>PGVERTDITYNLTSDIDAAAYLEELKQNPIINNKIMNPVGQCESLMTPVSNFMNEKGFDNIRYRGIFIWDKPTEEIPTNHFAVVGNKEGKDYVFDVSAHQFENRGMSNLNGPLILSADEWVCKYRMATRRKLIYYTDFSNSSIAANAYDALPRELESESMAGKVFVTSPRWFNTFKKQKYSLIGKM[2x]

SseI is secreted into host cells by Salmonella and contributes to the establishment of systemic infections. SseI (also called SrfH) is an SPI-2-translocated protein that has been directly linked to systemic infection. The C-terminal domain (∼140–322) of SseI contains its catalytic function and shows some sequence similarity (19% identity over a 88-amino-acid stretch) to Pasteurella multocida toxin (PMT or ToxA), which causes atrophic rhinitis in swine. Based on its structural matches, SseI is a member of a particular subgroup (clan CA) of the cysteine protease superfamily.

Crystals of reductively methylated SeMet-derivative and native forms of SseI (37–322) were grown as described and their structures were solved using SAD and molecular replacement, respectively. The native crystals diffracted to 2.05 Å resolution and belonged to a different space group (P212121) to the SeMet-derivative crystals (P41212). The native structure was solved using the SeMet-derivative structure as a starting model and showed two molecules of the protein per asymmetric unit. No density was observed for the first 12 and the last nine residues of each molecule. The dimer is linked by a disulfide bond between Cys258 of each chain on the opposite face of the molecule to the catalytic Cys176. The dimer is likely to be a crystal artifact since the C-terminal domain purifies as a monomer on size-exclusion chromatography. The SeMet protein was purified using 10 mM DTT instead of 2 mM DTT to prevent Se oxidation, which may explain why it did not crystallize as a disulfide-linked dimer under these reducing conditions. The chain backbone in the native structure did not show any large deviations from the SeMet-derivative structure, with r.m.s.d.s of 0.277 Å (chain A) and 0.250 Å (chain B) between the two models.>EFRPEMLQGKKVIVTGASKGIGREMAYHLAKMGAHVVVTARSKETLQKVVSHCLELGAASAHYIAGTMEDMTFAEQFVAQAGKLMGGLDMLILNHITNTSLNLFHDDIHHVRKSMEVNFLSYVVLTVAALPMLKQSNGSIVVVSSLAGKVAYPMVAAYSASKFALDG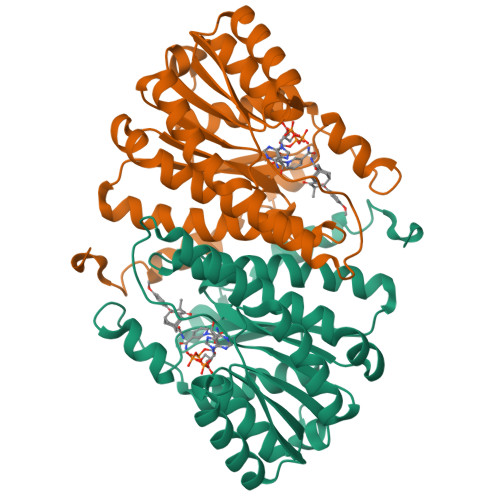FFSSIRKEYSVSRVNVSITLCVLGLIDTETAMKAVSGIVHMQAAPKEECALEIIKGGALRQEEVYYDSSLWTTLLIRNPSRKILEFLYSTSYNMDRF[8x]>[6x]SSQIRQNYSTEVEAAVNRLVNLYLRASYTYLSLGFYFDRDDVALEGVCHFFRELAEEKREGAERLLKMQNQRGGRALFQDLQKPSQDEWGTTLDAMKAAIVLEKSLNQALL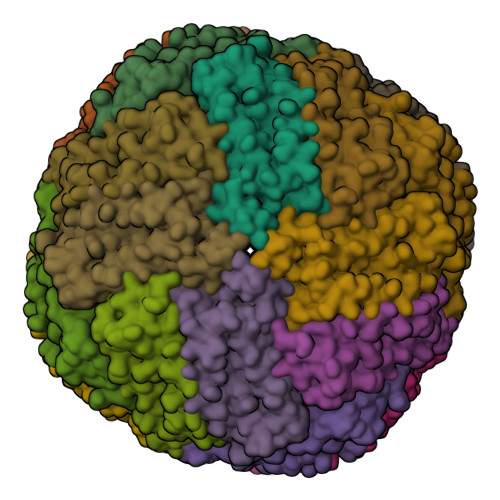DLHALGSAQADPHLCDFLESHFLDEEVKLIKKMGDHLTNIQRLVGSQAGLGEYLFERLTLKHD> GLEHHHHHHQDITELPFPVRQDSPLTEVLPTDLKTKDNFVARDPDLLRLTGSHPFNSEPPLTKLYDSGFLTPVSLHFVRNHGPVPYVPDENILDWEVSIEGMVETPYKIKLSDIMEQFDIYSTPVTMVCAGNRRKEQNMVKKGAGFNWGAAGTSTSLWTGCMLGDVIGKARPSKRARFVWMEGADNPANGAYGTCIRLSWCMDPERCIMIAYQQNGEWLHPDHGKPLRVVIPGVIGGRSVKWLKKLVVSDRP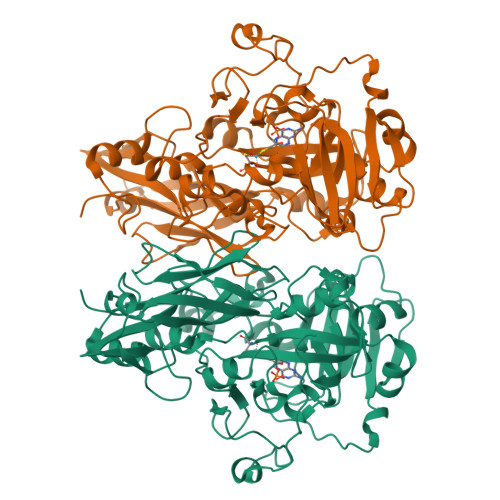SENWYHYFDNRVLPTMVTPEMAKSDDRWWKDERYAIYDLNLQTIICKPENQQVIKISEDEYEIAGFGYNGGGVRIGRIEVSLDKGKSWKLADIDYPEDRYREAGYFRLFGGLVNVCDRMSCLCWCFWKLKVPLSELARSKDILIRGMDERMMVQPRTMYWNVTSMLNNWWYRVAIIREGESLRFEHPVVANKPGGWMDRVKAEGGDILDNNWGEVDDTGQAG> MKLVNIWLLLLVVLLCGKKHLGDRLEKKSFEKAPCPGCSHLTLKVEFSSTVVEYEYIVAFNGYFTAKARNSFISSALKSSEVDNWRIIPRNNPSSDYPSDFEVIQIKEKQKAGLLTLEDHPNIKRVTPQRKVFRSLKYAESDPTVPCNETRWSQKWQSSRPLRRASLSLGSGFWHATGRHSSRRLLRAIPRQVAQTLQADVLWQMGYTGANVRVAVFDTGLSEKHPHFKNVKERTNWTNERTLDDGLGHGTFVAGVIASMRECQGFAPDAELHIFRVFTNNQVSYTSWFLDAFNYAILKKIDVLNLSIGGPDFMDHPFVDKVWELTANNVIMVSAIGNDGPLYGTLNNPADQMDVIGVGGIDFEDNIARFSSRGMTTWELPGGYGRMKPDIVTYGAGVRGSGVKGGCRALSGTSVASPVVAGAVTLLVSTVQKRELVNPASMKQALIASARRLPGVNMFEQGHGKLDLLRAYQILNSYKPQASLSPSYIDLTECPYMWPYCSQPIYYGGMPTVVNVTILNGMGVTGRIVDKPDWQPYLPQNGDNIEVAFSYSSVLWPWSGYLAISISVTKKAASWEGIAQGHVMITVASPAETESKNGAEQTSTVKLPIKVKIIPTPPRSKRVLWDQYHNLRYPPGYFPRDNLRMKNDPLDWNGDHIHTNFRDMYQHLRSMGYFVEVLGAPFTCFDASQYGTLLMVDSEEEYFPEEIAKLRRDVDNGLSLVIFSDWYNTSVMRKVKFYDENTRQWWMPDTGGANIPALNELLSVWNMGFSDGLYEGEFTLANHDMYYASGCSIAKFPEDGVVITQTFKDQGLEVLKQETAVVENVPILGLYQIPAEGGGRIVLYGDSNCLDDSHRQKDCFWLLDALLQYTSYGVTPPSLSHSGNRQRPPSGAGSVTPERMEGNHLHRYSKVLEAHLGDPKPRPLPACPRLSWAKPQPLNETAPSNLWKHQKLLSIDLDKVVLPNFRSNRPQVRPLSPGESGAWDIPGGIMPGRYNQEVDYKDDDDKGSDYKDDDDKGSDYKDDDDK;> METDTLLLWVLLLWVPGSTGDKQEERAVRDRNLLQVHDHNQPIPWKVQFNLGNSSRPSNQCRNSIQGKHLITDELGYVCERKDLLVNGCCNVNVPSTKQYCCDGCWPNGCCSAYEYCVSCCLQPNKQLLLERFLNRAAVAFQNLFMAVEDHFELCLAKCRTSSQSVQHENTYRDPIAKYCYGESPPELFPAHHHHHHHHHH

Site-one protease (S1P, also known as Membrane-bound transcription factor site-1 protease (MBTPS1), or Subtilisin kexin isozyme 1 (SKI-1)), is a membrane-bound protease that mediates the proteolytic activation of transcription factors, hormones, and enzymes required for lipogenesis, the endoplasmic reticulum (ER) stress response, and lysosomal biogenesis, among others. A zymogen serine protease, S1P matures through autoproteolysis of two pro-domains, with one cleavage event in the endoplasmic reticulum (ER) and the other in the Golgi. We recently identified the SREBP regulating gene, (SPRING), which enhances S1P maturation and is necessary for SREBP signaling. SPRING activates S1P by dislodging its inhibitory pro-domain and stabilizing intra-domain contacts.

We determined the structure of the SPRINGecto-S1Pecto complex to 2.3 Å using cryo-electron microscopy (cryo-EM). The Peptidase S8 protease harbors a catalytic triad of D218, H249, and S414 and the oxyanion hole residue N3383,16. We did observe density for a putative calcium molecule in the GIFT subdomain within an acidic pocket near the GIFT-Protease interface. Our cryo-EM map for S1Pecto-SPRINGecto shows density for a 7-sugar tree at S1P N515, the form of N-linked glycan that is homogenously produced in HEK GnTI- cells. SPRINGecto presents a cysteine-rich fold that we term the Cysteine-rich enabler of S1P activity (CREST) domain (residues 36-205). The final model for SPRINGecto contains residues 76–138 and residues 165–196. SPRINGecto makes protein-protein contacts with all three subdomains of C-form S1Pecto and the total binding surface between S1Pecto and SPRINGecto is ~1200 Å2. SPRINGecto binds a somewhat hydrophobic ridge beginning at the GIFT subdomain, running along the protease, and terminating at the P-like subdomain. In contrast, S1Pecto co-expressed with SPRINGecto forms a stable heterodimeric complex lacking the cleaved S1P A-domain and efficiently cleaves an exogenous SREBP2 peptide.> RSPPAPPLPQRPLSPLHPLGCNDSEVLAVAGFALQNINRDQKDGYMLSLNRVHDVREHYQEDMGSLFYLTLDVLETDCHVLSRKAQKDCKPRMFYESVYGQCKAMFHINKPRRVLYLPAYNCTLRPVSKRKTHTTCPDCPSPIDLSNPSALEAATESLAKFNSKSPSKKYELVKVTKAMNQWVSGPAYYVEYLIKEAPCTKSQASCSLQHSDSEPVGICQGSTVQSSLRHVPLIQPVEKSVTVTCEFFESQAQVPGDENPAVTQGPQKLPQKNTAPTS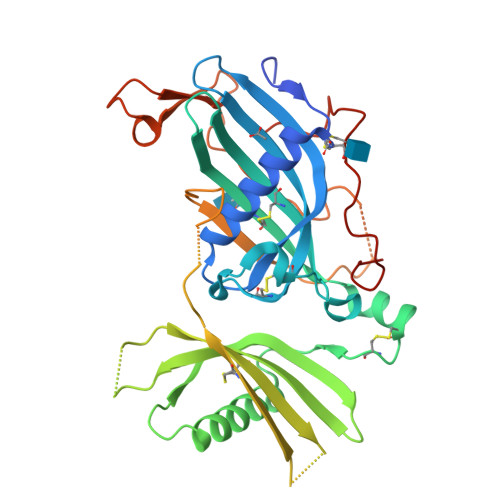SPSVTAPRGSIQHLPELDDEKPEESKGGSPEEAFPVQLDLTTNPQGDTLDVSFLYLEPGDKKLVVLPFPGKEQRSAECPGPEKENNPLVLPPLEHHHHHH Nuclear respiratory factor 1 (NRF1) regulates the expression of genes that are vital for mitochondrial biogenesis, respiration, and various other cellular processes. NRF1 was initially identified as a transcription activator of cytochrome c by binding to the cytochrome c promoter as a homodimer. Subsequently, a consensus sequence GCGCNTGCGC (N represents any nucleotide) was identified as the DNA binding motif of NRF1 (6), which has also been detected in the promoters of many other nuclear genes relevant to mitochondrial biogenesis and respiration, such as the promoters of reductase (ubiquinone-binding protein) complex (6), cytochrome oxidase assembly factor COX17 (7), myocyte enhancer factor 2A (MEF2A), and ferridoxin reductase (FDXR). Our structural, mutagenesis and luciferase reporter assay results revealed that, although the NRF1 DBD alone is capable of recognizing the TGCGC DNA motif, the cooperativity between DD and DBD is essential for the binding of the intact GCGCATGCGC sequence and the transcriptional activity of NRF1.

To investigate the molecular mechanisms underlying the selective binding of NRF1 to the GCGCATGCGC DNA sequence, we determined the crystal structure of NRF1 (aa 54–284) with a 14pb ATGCGCATGCGCAT dsDNA. In the complex structure, NRF1 forms a homodimer and binds to a single ATGCGCATGCGCAT DNA duplex. The β1 and β2 strands from each monomer form an intermolecular 4-stranded β-sheet, while the α3 and α4 helices from two monomers form antiparallel helices and pack against either side of the β-sheet through extensive hydrophobic interactions. The DBD is composed of three helices α5 to α7 and two short 310-helix, and each DBD possesses positively charged surfaces to recognize two neighboring major grooves of the DNA duplex from nearly opposite side. Interestingly, in the NRF1 dimer-dsDNA complex, although the DD or DBD from the two monomers superimposes very well (with RMSDs of 0.33Å and 0.34Å, respectively), the arrangement of these two domains differs in both monomers. When binds with DNAs, only one NRF1 monomer adopts a structural conformation that is close to the AlphaFold2 predicted model, and the DBD and DD of the other NRF1 monomer adopts a U-turn conformation, resulting in the two DBDs of the NRF1 homodimer bind to the consensus sequence GCGCNTGCGC from nearly the opposite side of the DNA duplex. In the NRF1 dimer-dsDNA complex, two DBDs of the NRF1 dimer bind to the DNA duplex from opposite directions. Hence, residues R206, N242, and R244 of NRF1 DBD are critical in sequence-specific binding to the GCGCATGCGC motif. Remarkably, the helix α3 from the DD of the NRF1 monomer1 exhibits a positively charged surface and forms electrostatic interaction with the DNA duplex.

>GDDSDILNSTAADEVTAHLAAAGPVGMAAAAAVATGKKRKRPHVFESNPSIRKRQQTRLLRKLRATLDEYTTRVGQQAIVLCISPSKPNPVFKVFGAAPLENVVRKYKSMILEDLESALAEHAPAPQEVNSELPPLTIDGIPVSVDKMTQAQLRAFIPEMLKYSTGRGKPGWGKESCKPIWWPEDIPWANVRSDVRTEEQKQRVSWTQALRTIVKNCYKQHGREDLLYAFED[2x]> MSANSLLGSLRELQVLVLNPPGEVSDALVLQLIRIGCSVRQCWPPPEAFDVPVDVVFTSIFQNRHHDEIAALLAAGTPRTTLVALVEYESPAVLSQIIELECHGVITQPLDAHRVLPVLVSARRISEEMAKLKQKTEQLQDRIAGQARINQAKVLLMQRHGWDEREAHQHLSREAMKRREPILKIAQEL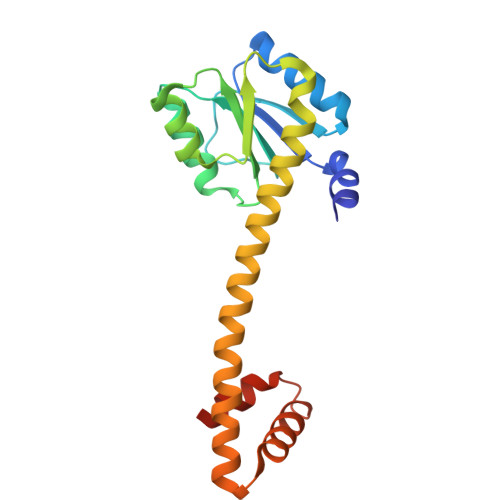LGNEPSA>MIAHLINTDIGNRGVLKVYLDYRRKNFNFLHNSTKMFLDNLERVLIVTGFPIPPMMVAETDGPPGALAIYRAVEMLGGKAEILTYSEVEKALEPFGVSLARTPEPEDYSLIISVETPGRAADGRYYSMSALEIKRDPLDGIFLKARALGIPTIGVGDGGNEIGMGKIRELVVGHVPHGEKIASVVETDELIVSAVSNWGAYGLVAQASIEVGRNLLEGWDERRVIEAISSAGLIDGVSKTLAPSVDGIRLMVHEGIVELLKAVVDEAIKL[6x]

Here, it is reported that multiple zinc ions can easily be charged onto the surface of proteins with no intrinsic zinc-binding site by using zinc-containing solutions. Here, we show that the surface of proteins can be charged with zinc ions and that the anomalous signals from these zinc ions can be used for structure determination of proteins. In conclusion, we demonstrated that protein crystals grown in the presence of zinc ions or soaked in a zinc-containing solution are easily charged with multiple zinc ions on the protein surface and that they are suitable for zinc SAD/MAD phasing. Considering the high phasing effectiveness and multiple zinc-binding sites, we believe that zinc derivatization of the protein surface is a largely unnoticed but promising method for phase determination of protein crystals.

Recently, we obtained crystals of TON_0340 in a precipitant solution containing zinc acetate. Based on our confidence in zinc derivatization and phase determination, we collected a 2.3 Å resolution SAD data set from a crystal that was cooled in a cryostream at 100 K after briefly being immersed in a cryoprotectant solution consisting of 20% glycerol, 5%(v/v) 2-propanol, 100 mM sodium acetate pH 5.0, 350 mM zinc acetate. The TON_0340 crystals, which contained six molecules per asymmetric unit, belonged to the tetragonal space group P43212, with unit-cell parameters a = b = 107.44, c = 355.03 Å. According to the plot of 〈d″/sig〉 versus resolution, zinc anomalous signal was present, although it decreased drastically at high resolution. Additionally, three zinc ions bound to a cluster of six acidic residues were located in a putative active-site cleft.>[4x]MSVEGLGKDFCGAIIPDNFFPIEKLRNYTQMGLIRDFAKGSAVIMPGEEITSMIFLVEGKIKLDIIFEDGSEKLLYYAGGNSLIGKLYPTGNNIYATAMEPTRTCWFSEKSLRTVFRTDEDMIFEIFKNYLTKVAYYARQVAEMNTYNPTIRILRLFYELCSSQGKRVGDTYEITMPLSQKSIGEITGVHHVTVSRVLASLKRENILDKKKNKIIVYNLGELKHLSEQTSYYSDPNSSSVDKLAAALDHH

The transcriptional regulator CprK from Desulfitobacterium spp. induces expression of halorespiratory genes upon binding of o-chlorophenol ligands and is reversibly inactivated by oxygen through disulphide bond formation. The CprK associated with the o-chlorophenolacetic acid (OCPA) reductive dehalogenase (CprAB) from D. dehalogenans and the closely related D. hafniense has been shown to bind OCPA with μM affinity leading to sequence-specific DNA-binding, and ultimately transcriptional activation of the associated cpr gene cluster (Pop et al., 2004; 2006; Gabor et al., 2006; Joyce et al., 2006; Mazon et al., 2007). Members of this family are homodimeric and contain an N-terminal sensor domain linked via a long α-helix (involved in formation of the dimer interface) to the C-terminal helix–turn–helix (HTH) DNA-binding domain. We here present crystal structures of the oxidized ligand-free (3.2 Å) and reduced ligand-free (2.0 Å), OCPA-bound (1.8 Å) and DNA-bound (1.8 Å) D. hafniense CprK in addition to an intermediate OCPA-bound structure obtained by soaking ligand-free crystals (2.0 Å).

In order to avoid formation of the inactive, oxidized CprK under aerobic conditions, the CprKC200S mutant was used to obtain structural insights into the reduced CprK structure. Previous studies indicated that this mutation does not significantly affect CprK function and only has minor impact on DNA-binding affinity. The 1.8 Å crystal structure of the CprK:OCPAC200S complex contains two CprK dimers in the asymmetric unit, each dimer binding two OCPA ligands to the N-terminal sensor domains. Similar to the previously determined oxidized CprK:OCPA complex, the phenol and acetic acid groups of OCPA interact with amino acids from both CprK monomers through extended hydrogen bonding networks. This positions the chloride atom within a hydrophobic pocket at the dimer interface (Joyce et al., 2006). In contrast to the marked asymmetry of the oxidized CprK:OCPA structure, near-perfect twofold symmetry relates the monomer structures within a single CprKC200S:OCPA dimer. This arrangement places both HTH domains in a position compatible with binding to the palindromic (de)halobox DNA. The CprKC200S:OCPA dimer structure reveals that each individual CprK DNA-binding domain establishes a small contact area [approximately 270 Å2 with a surface complementarity of 0.691] with both N-terminal domains of the dimer. A large proportion of this contact area is centred around an extensive salt-bridge network established between the DNA-binding domain Arg-155 and Glu-159 with the central α-helix Arg-139 and Glu-143 residues in addition to Glu-68 (in the sensor domain). In contrast, a significant set of hydrophobic interactions is established within each single monomer between residues Ile-14–Ile-15–Pro-16 from the N-terminus and the DNA-binding domain that leads to near-complete burial of both Ile side-chains.> MEIAFLLNGETRRVRIEDPTQSLLELLRAEGLTGTKEGCNEGD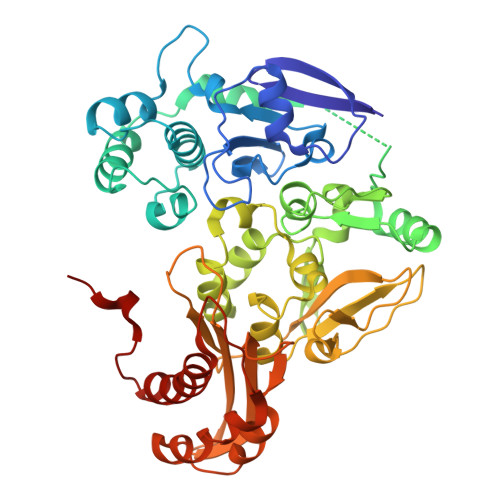CGACTVMIRDAAGSRAVNACLMMLPQIAGKALRTIEGIAAPDGRLHPVQQAMIDHHGSQCGFCTPGFIVSMAAAHDRDRKDYDDLLAGNLCRCTGYAPILRAAEAAAGEPPADWLQADAAFTLAQLSSGVRGQTAPAFLPETSDALADWYLAHPEATLIAGGTDVSLWVTKALRDLPEVAFLSHCKDLAQIRETPDGYGIGAGVTIAALRAFAEGPHPALAGLLRRFASEQVRQVATIGGNIANGSPIGDGPPALIAMGASLTLRRGQERRRMPLEDFFLEYRKQDRRPGEFVESVTLPKSAPGLRCYKLSKRFDQDISAVCGCLNLTLKGSKIETARIAFGGMAGVPKRAAAFEAALIGQDFREDTIAAALPLLAQDFTPLSDMRASAAYRMNAAQAMALRYVRELSGEAVAVLEVMP>[4x]MTHELISLPYAVDALAPVISKE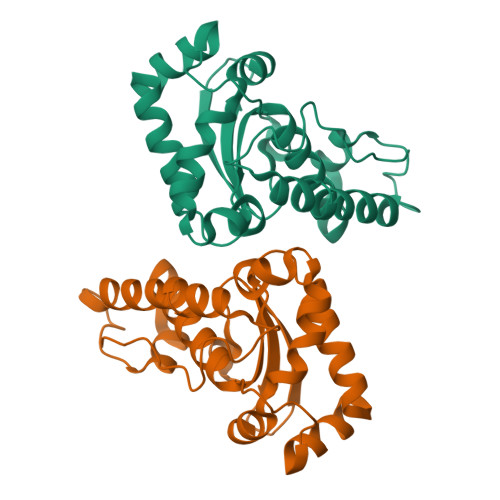TVEFHHGKHLKTYVDNLNKLIIGTEFENADLNTIVQKSEGGIFNNAGQTLNHNLYFTQFRPGKGGAPKGKLGEAIDKQFGSFEKFKEEFNTAGTTLFGSGWVWLASDANGKLSIEKEPNAGNPVRKGLNPLLTFDVWEHAYYLTYQNRRADHLKDLWSIVDWDIVESRY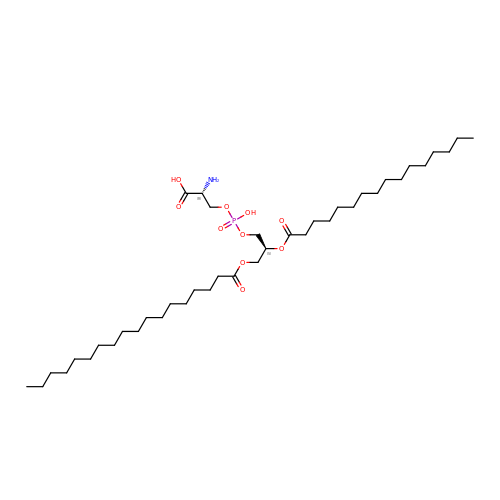O-[(R)-[(2S)-2-(hexadecanoyloxy)-3-(octadecanoyloxy)propoxy](hydroxy)phosphoryl]-D-serine | C40 H78 N O10 P | WZFUPCSEUKNOBF-PQQNNWGCSA-N> M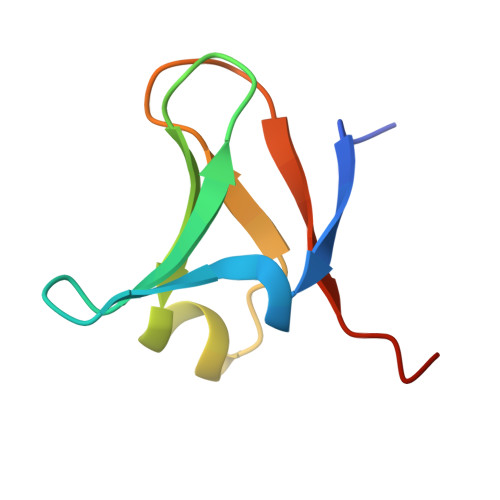STYDEIEIEDMTFEPENQMFTYPCPCGDRFQIYLDDMFEGEKVAVCPSCSLMIDVVHHHHHH>MKETNFGEKTRVLVVGGTGSLGRRIVSACLAEGHETYVLQRPEIGVDIEKVQLLLSFKRLGAHLVEGSFSDHQSLVSAVKQVDVVVSAMSGVHFRTHNIPVQLKLVAAIKEAGNVKRFLPSEFGMDPSRMGHAMPPGSETFDQKMEIRNAIKAAGISHTYLVGACFAAYFGGNLSQMGTLFPPKNKVDIYGDGNVKVVFVDEDDMAKYTAKTLNDPRTLNKTVYVRPTDNILTQMELVQIWEKLTEKELEKTYVSGNDFLADIEDKEISHQAGLGHFYHIYYEGCLTDHEVGDDEEATKLYPDVKYKRMDEYLKIFV[2x]

Pinoresinol/lariciresinol reductase (PLR), an NADPH-dependent reductase, converts pinoresinol to lariciresinol and subsequently to secoisolariciresinol. Here, we present crystal structures of IiPLR1 from Isatis indigotica and pinoresinol reductases (PrRs) AtPrR1 and AtPrR2 from Arabidopsis thaliana, in the apo, substrate-bound and product-bound states. The crystal structures were captured in the apo, substrate-bound and/or product-bound forms. We found that, for all 16 structures we solved, each enzyme adopts a similar head-to-tail dimer conformation, strongly suggesting that each PLR/PrR functions as a homodimer, consistent with the literature that TpPLR1 exists as a dimeric entity in solution. Each structure contains a head-to-tail homodimer, and the catalytic pocket comprises structural elements from both monomers. β4 loop covers the top of the pocket, and residue 98 from the loop governs catalytic specificity.

Intriguingly, the β4 loop is well defined in the AtPrR1_NAP structure but disordered in the AtPrR1/2_apo structures. These structural differences suggest that the loops are somewhat flexible, and act as a switch to control the binding of NADPH and release of NADP+. Similar conformational changes of β2 loop and α10-helix can be seen by comparing the structure of AtPrR1_NAP_ + PIN with that of AtPrR1_NAP and the structure of AtPrR2_NAP_ + PIN with that of AtPrR2_apo.> 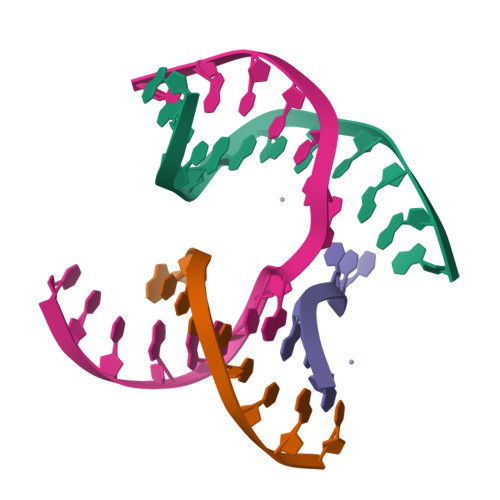GAGCAGACCAGA;> CGTCACTCA;> TCTACG;> TCTGAGTGGGTCTGC>[2x]MPIHIGSSIPLMVEKMLTEMVKPSKHIPQQTLNLSTLDNDPYNE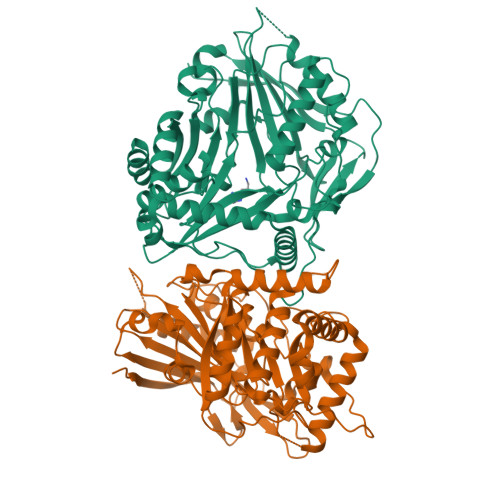VIYKACYVFKAKNVADDDNRPEALLREALSDLLGYYYPLSGSLKRQESDRKLQLSCGGDGGGVPFTVATANVELSSLKNLENIDSDTALNFLPVLHVDIDGYRPFALQVTKFECGGFILGMAMSHAMCDGYGEGHIMCALTDLAGGKKKPMVTPIWERERLVGKPEDDQPPFVPGDDTAASPYLPTDDWVTEKITIRADSIRRLKEATLKEYDFSNETITTFEVIGAYLWKSRVKALNLDRDGVTVLGLSVGIRNVVDPPLPDGYYGNAYIDMYVPLTAREVEEFTISDIVKLIKEAKRNAHDKDYLQEELANTEKIIKMNLTIKGKKDGLFCLTDWRNIGIFGSMDFGWDEPVNIVPVVPSETARTVNMFMRPSRLESDMVGGVQIVVTLPRIAMVKFKEEMEALE>LGRHFYVTGPVVRGAGRGGKELGFPTANQYFHDTVALPADGVYAGWLTILPTEAPVSGNMEPEVAYAAAISVGTNPTFGDEQRSVESFVLDRDADLYGHDVKVEFVDHVRAMEKFDSVEQLLEVMAKDVQKTRTLLAQDVQ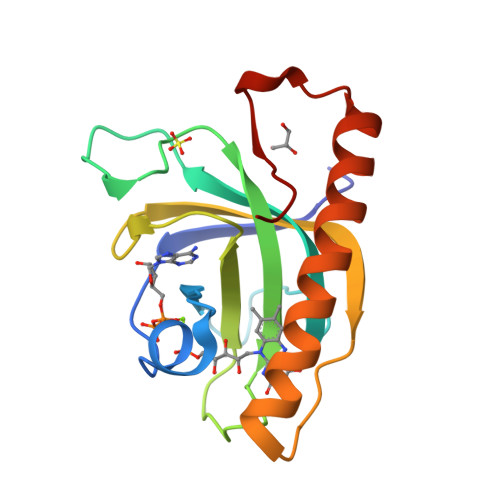AHKMAPETYFLQAES[2x]>[2x]MAHNHRHKHADYKDDDDKKLNSATSADEQPHIGNYRLLKTIGKGNF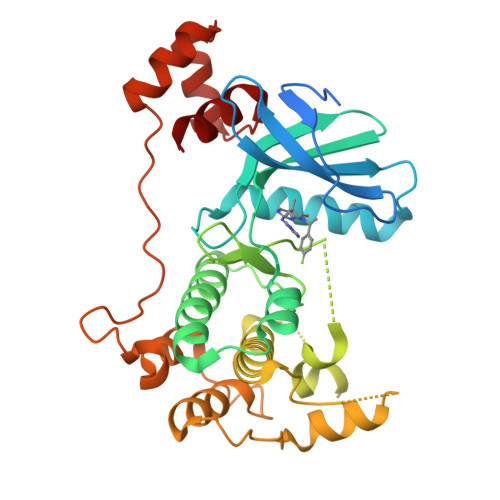AKVKLARHILTGKEVAVKIIDKTQLNSSSLQKLFREVRIMKVLNHPNIVKLFEVIETEKTLYLVMEYASGGEVFDYLVAHGRMKEKEARAKFRQIVSAVQYCHQKFIVHRDLKAENLLLDADMNIKIADFGFSNEFTFGNKLDTFCGSPPYAAPELFQGKKYDGPEVDVWSLGVILYTLVSGSLPFDGQNLKELRERVLRGKYRIPFYMSTDCENLLKKFLILNPSKRGTLEQIMKDRWMNVGHEDDELKPYVEPLPDYKDPRRTELMVSMGYTREEIQDSLVGQRYNEVMATYLLLGYK>[2x]PNFSGNWKIIRSENFEELLKVLGVNVMLRKIAVAAASKPAVEIKQE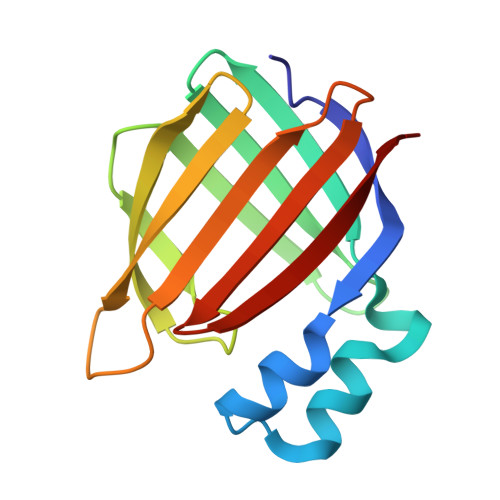GDTFYIKTSTTVRTTEINFKVGEEFEEQTVDGRPCKSLVKWESENKMVCEQKLLKGEGPKTSWTLELTNDGELIDTMTADDVVCTKVFVRE In this light, new lines of evidence point to a crucial role of the cytochrome bd oxidase for mycobacterial pathophysiology. This quinol-oxidizing terminal oxygen reductase is encoded by the cydAB gene cluster and is a central component of the branched respiratory chain of M. tuberculosis. During infection and proliferation, the cytochrome bd oxidase plays a crucial role for mycobacterial pathophysiology by maintaining aerobic respiration at limited oxygen concentrations. The cyt. bdMtb is structurally characterized by the presence of a pseudo-symmetrical heterodimer formed by CydA and CydB. The CydA subunit represents the catalytically active component of the enzyme complex, harboring the three prosthetic heme groups, and the quinol binding and oxidation domain (Q-loop).

Cofactor assembly and oxygen reductase activity were validated via UV–Vis spectroscopy and oxygen consumption measurements. The three-dimensional structure of POPC nanodisc reconstituted cyt. bdMtb, in the as isolated mixed-valence state was determined by single-particle electron cryo-microscopy (cryo-EM) to a resolution of 2.5 Å. Despite the close structural similarity to the cytochrome bd oxidase from Escherichia coli (cyt. bdEcoli), the absence of a CydX subunit homolog neither affects cofactor assembly of cyt. bdMtb, nor does it influence cofactor composition as shown by our cryo-EM structure and spectroscopic data. The cavity that harbors a stabilizing UQ-8 molecule in cyt. bdE.coli is absent in cyt. bdM.tb. Instead, we identify a series of Trp and Phe residues that occupy this space. They form stabilizing van-der-Waals contacts between TMHs 3, 4, 5, and 8 that render the structural quinone unnecessary. A distinguishing feature of the mycobacterial Q-loop is the presence of a disulfide bond between Cys266.A and Cys285.A within the QN region exposed towards the periplasmic space. Our simulations demonstrate that the disulfide bond rigidifies the disordered Q-loop segment and reduces flexibility between QN and Qh1. We conclude that the confined conformation of the QN-region sterically hinders an interaction between substrate molecules and the highly conserved Glu263.A which is involved in quinol binding and oxidation in immediate proximity to heme b55816. In proximity to the disulfide bond, within the cleft formed between TMH 1 and 9 we identified a bound menaquinone-9 (MK-9) molecule. The local environment that forms this previously unknown MK-9 binding pocket is composed of the heme b595 porphyrin scaffold, Arg8.A and Trp9.A of TMH1, and Met397.A of TMH 9.

> MNVVDISRWQFGITTVYHFIFVPLTIGLAPLIAVMQTLWVVTDNPAWYRLTKFFGKLFLINFAIGVATGIVQEFQFGMNWSEYSRFVGDVFGAPLAMEGLAAFFFESTFIGLWIFGWNRLPRLVHLACIWIVAIAVNVSAFFIIAANSFMQHPVGAHYNPTTGRAELSSIVVLLTNNTAQAAFTHTVSGALLTAGTFVAAVSAWWLVRSSTTHADSDTQAMYRPATILGCWVALAATAGLLFTGDHQGKLMFQQQPMKMASAESLCDTQTDPNFSVLTVGRQNNCDSLTRVIEVPYVLPFLAEGRISGVTLQGIRDLQQEYQQRFGPNDYRPNLFVTYWSFRMMIGLMAIPVLFALIALWLTRGGQIPNQRWFSWLALLTMPAPFLANSAGWVFTEMGRQPWVVVPNPTGDQLVRLTVKAGVSDHSATVVATSLLMFTLVYAVLAVIWCWLLKRYIVEGPLEHDAEPAAHGAPRDDEVAPLSFAY;> MVLQELWFGVIAALFLGFFILEGFDFGVGMLMAPFAHVGMGDPETHRRTALNTIGPVWDGNEVWLITAGAAIFAAFPGWYATVFSALYLPLLAILFGMILRAVAIEWRGKIDDPKWRTGADFGIAAGSWLPALLWGVAFAILVRGLPVDANGHVALSIPDVLNAYTLLGGLATAGLFSLYGAVFIALKTSGPIRDDAYRFAVWLSLPVAGLVAGFGLWTQLAYGKDWTWLVLAVAGCAQAAATVLVWRRVSDGWAFMCTLIVVAAVVVLLFGALYPNLVPSTLNPQWSLTIHNASSTPYTLKIMTWVTAFFAPLTVAYQTWTYWVFRQRISAERIPPPTGLARRAP>[2x]AEAGITGTWYNQLGSTFIVTAGADGALTGTYEAAVGNAESRYVLTGRYDSAPATDGSGTALGWTVAWKNNYRNA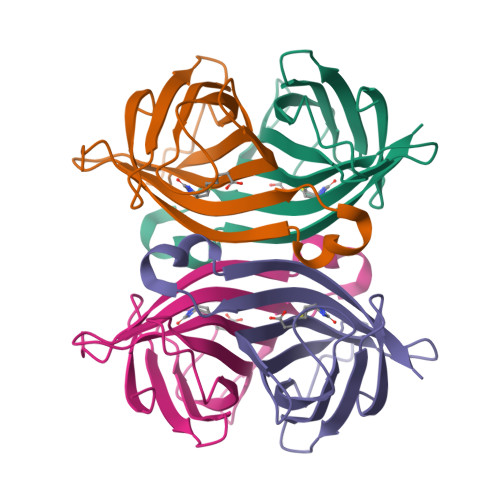HSATTWSGQYVGGAEARINTQWLLTSGTTEANAWKSTLVGHDTFTKVKPSAAS> GPGSEFMDGPGASAVVVRVGIPDLQQTKCLRLDPTAPVWAAKQRVLCALNHSLQDALNYGLFQPPSRGRAGKFLDEERLLQDYPPNLDTPLPYLEFRYKRRVYAQNLIDDKQFAKLHTKANLKKFMDYVQLHSTDKVARLLDKGL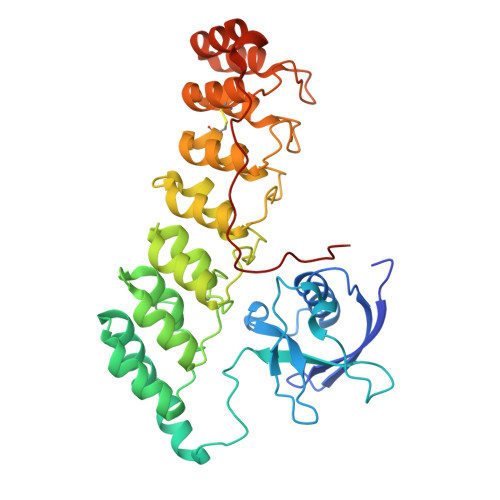DPNFHDPDSGECPLSLAAQLDNATDLLKVLRNGGAHLDFRTRDGLTAVHCATRQRNAGALTTLLDLGASPDYKDSRGLTPLYHSALGGGDARCCELLLHDHAQLGTTDENGWQEIHQACRFGHVQHLEHLLFYGANMGAQNASGNTALHICALYNQESCARVLLYRGANKDVRNYNSQTAFQVAIIAGNFELAEVIKTHKDSDVVPFRETPSYAKRRRLAGPSGLASPR>[2x]SMEAPTRIRDTPEDIVLEAPASGLAFHPARDLLAAGDVDGDVFVFSYSCQEGETKELWSSGHHLKACRAVAFSEDGQKLITVSKDKAIHVLDVEQGQLERRVSKAHGAPINSLLLVDENVLATGDDTGGIRLWDQRKEGPLMDMRQHEEYIADMALDPAKKLLLTASGDGCLGIFNIKRRR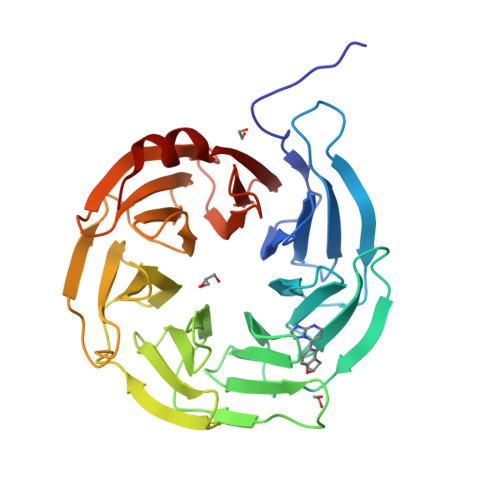FELLSEPQSGDLTSVTLMKWGKKVACGSSEGTIYLFNWNGFGATSDRFALRAESIDCMVPVTESLLCTGSTDGVIRAVNILPNRVVGSVGQHTGEPVEELALSHCGRFLASSGHDQRLKFWDMAQLRAVVVDD> AETADLSASVPTRPAEPERKTLADYGGYPSALDAVKQKNDAAVAAYLENAGDSAMAENVRNEWLKSLGARRQWTLFAQEYAKLEPAGRAQEVECYADSSRNDYTRAAELVKNTGKLPSGCTKLLEQAAASGLLDGNDAWRRVRGLLAGRQTTDARNLAAALGSPFDGGTQGSREYALLNVIGKEARKSPNAAALLSEMESGLSLEQRSFAWGVLGHYQSQNLNVPAALDYYGKVADRRQLTDDQIEWYARAALRARRWDELASVISHMPEKLQKSPTWLYWLARSRAATGNNQEAEKLYKQAAATGRNFYAVLAGEELGRKIDTRNNVPDAGKNSVRRMAEDGAVKRALVLFQNSQSAGDAKMRRQAQAEWRFATRGFDEDKLLTAAQTAFDHGFYDMAVNSAERTDRKLNYTLRYISPFKDTVIRHAQNVNVDPAWVYGLIRQESRFVIGAQSRVGAQGLMQVMPATAREIAGKIGMDAAQLYTADGNIRMGTWYMADTKRRL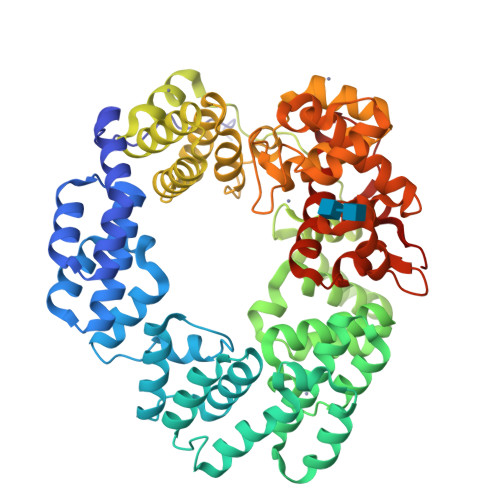QNNEVLATAGYNAGPGRARRWQADTPLEGAVYAETIPFSETRDYVKKVMANAAYYAALFGAPHIPLKQRMGIVPAR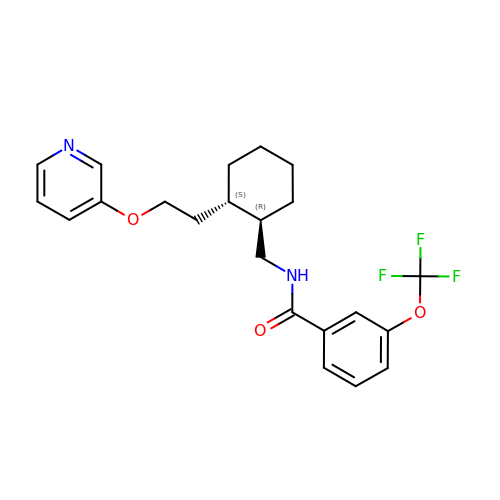N-{[(1R,2S)-2-{2-[(pyridin-3-yl)oxy]ethyl}cyclohexyl]methyl}-3-(trifluoromethoxy)benzamide | C22 H25 F3 N2 O3 | IERBKCIYEFEAOR-WMZOPIPTSA-N> RSCIDT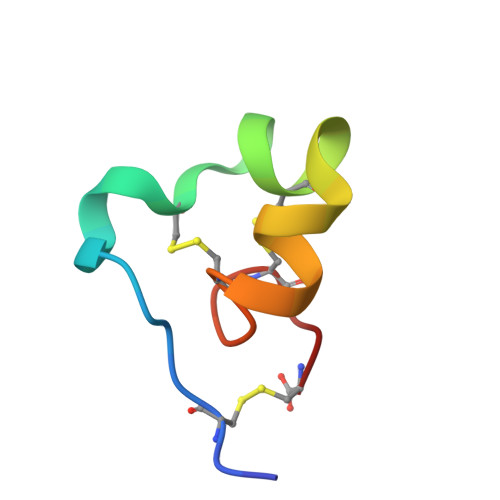IPKSRCTAFQCKHSMKYRLSFCRKTCGTC> AGARLPDLKIEKLEEGVYVHTSFEEVNGWGVVSKHGLVVLVNTDAYLIDTPFTATDTEKLVNWFVERGYKIKGTISSHFHSDSTGGIEWLNSQSI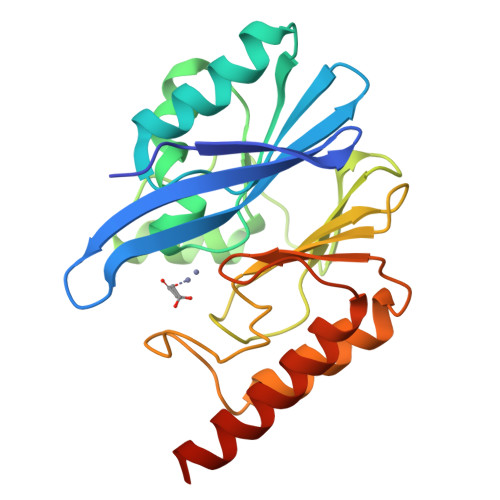PTYASELTNELLKKDGKVQAKNSFSGVSYWLVKNKIEVFYPGPGHTQDNVVVWLPEKKILFGGCFVKPDGLGNLGDANLEAWPKSAKILMSKYVKAKLVVSSHSEIGDASLLKRTWEQAVKGLNESKKPSQPSN>[14x]MSQTLLV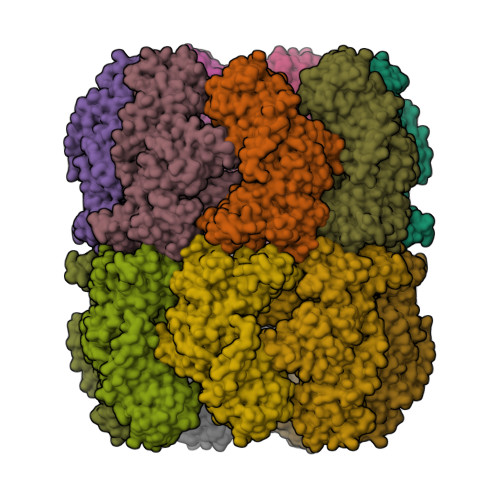HGKDAQGIIKQVLSEVYDAVTSTMGPNGQLVMIKNGVSTKTTKDGVTVARSIRFADEAHELVNRVITEPATKTDEECGDGTTTTIMLTHALYHLFKDFPGFQHHRNIEDLVERVIQRLESMAIRVEVDDPRLYQVALTSSNQDEKLARLVSELYANNKGSYPDIELKEGVNFEDQIEQTTGRTIRMFYANPWFAKGHQGGVTELTGFTAFVIDRRIDKEDTQKLIDGVNHLVKTHKQHLALPILLIARSFEEAANSTLMQLNAAHPTLVEDGRPWLIPLSTPVGGAIGTSELQDIAVMLNAPMLSDVADLTKLDTHSINGQHGQLELGGNRSILKSTTPKDEDRIEQHARGIEELLEGFSLSDKFSVRARYNERRIRTLRGKLITISVGGETYSEVKERVDRYEDVVKAIRSALENGILPGGGVSLVKAVFGTIKEGLEDKDQSAEFAKRYINSGIANELMRLSTIQHKLLFKDTALYKENGSFHFNDDWLNTPTVMNLATGEIGTPEGLGIYDTAYASITALKGGLQTAKILATTKTLILGEKLSAVKVR> TENILRKSDEEIQKEITARVKALESMLIEQGILTTSMIDRMAEIYENEVGPHLGAKVVVKAWTDPEFKKRLLADGTEACKELGIGGLQGEDMMWVENTDEVHHVVVCTLCSCYPWPVLGLPPNWFKEPQYRSRVVREPRQLLKEEFGFEVPPSKEIKVWDSSSEMRFVVLPQRPAGTDGWSEEELATLVTRE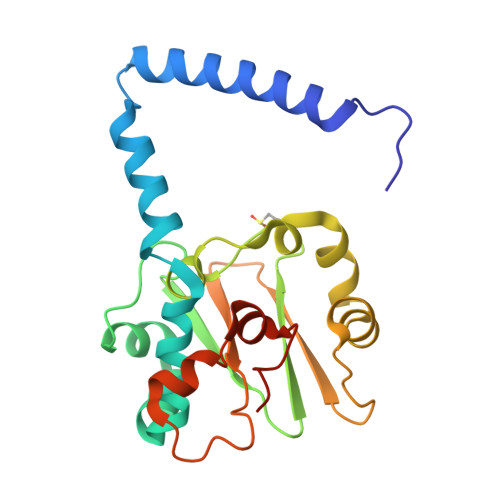SMIGVEPAKAVHHHHHH One of the proteins identified in these studies was classified as BTA121. While BTA121 does not share appreciable sequence similarity to any known protein domains or motifs, its N-terminal region is enriched in proline, glycine, and glutamic acid and contains a potential procyclic acidic repetitive protein (PARP) domain that was previously reported as having roles in Trypanosoma brucei survival and successful replication in its insect vector, the tsetse fly. BTA121 is a completely helical protein separated into an N-terminal and a C-terminal helical bundle. BTA121 does not share structural similarity with known proteins, and has the characteristic palmitate-binding cavity observed in tablysin-15, and palmitate binding was confirmed in vitro.

Recombinant BTA121 was produced and the crystal structure of BTA121 was solved using Se-SAD phasing. The final refined structure was obtained by phase extension by molecular replacement into the 2.8 Å resolution data collected at 1.000 Å wavelength. A total of 548 amino acid residues and 13 sulfate ions have ordered electron density  forming  a dimer. The first 91 amino acids of BTA121 and N-terminal putative PARP domain are disordered for each monomer. The monomer can also be viewed as having four helical domains (D1, 164–214; D2, 215–299; D3, 300–344; and D4, 345–435). Domains D1 and D2 are in the N-terminal bundle while D3 and D4 are in the C-terminal bundle. There are two possible crystallographic dimers; dimer 1 has an interface of parallel helices; while dimer 2 interfaces through loops. The interactions at the dimer 1 interface are hydrophobic and have a palindromic sequence. BTA121 has a network of interconnected tunnels connecting the large cavities some of which contain sulfate ions from the crystallization solution. The channels and tunnels connect all the cavities containing sulfate ions. The presence of such an extensive network of tunnels and cavities suggests that BTA121 may bind small molecular weight ligands, including lipids.

>SGVRPESGVGPESGVGPEAGVGPEAGVGPESGVGPEAGVGPEAGVGPESGVGPESGVGPEAGVRPEAGVRPEAGAGTDTETEEEIEEVVGDEEALAYLNETVIDPKLIALLDDFGVSRSGRKAISYIQGNLTSDVIYDRLNKLGADVVIEKIIKPTVSLLKTKGEALKIIEDPTNEGVKTRLQNMCKRYDGLVKGIGYDFFHGSIGTDRFAQAVVYYAPRFRKFKEIVKNPRVMDDIYGWLDADDRATINEIGKIVINATYDKDKFNNVLNSVGVYYVVRMIDIYRGVKIEHDEALNAITTVPDGVVKQDLQARLNRFKGEYYSNIRGTFKGFTDGLHFQIMTDGDKYRNYFIILKFDAQAARVAKARGATGSGS[2x]> GPLGSSLFNSEEDVVKMSPLPTVENQFTPTTAWSTSVGSGIGNFYSNLHPALADNVVYAADRAGLVKALNADDGKEIWSVSLAEKDGWFSKEPALLSGGVTVSGGHVYIGSEKAQVYALNTSDGTVAWQTKVAGEALSRPVVSDGLVLIHTSNGQLQALNEADGAVKWTVNLDMPSLSLRGESAPTTAFGAAVVGGDNGRVSAVLMEQGQMIWQQRISQATGSTEIDRLSDVDTTPVVVNGVVFALAYNGNLTALDLRSGQIMWKRELGSVNDFIVDGNRIYLVDQNDRVMALTIDGGVTLWTQSDLLHRLLTS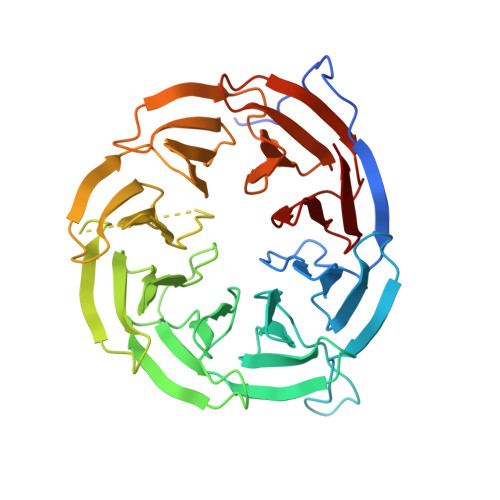PVLYNGNLVVGDSEGYLHWINVEDGRFVAQQKVDSSGFQTEPVAADGKLLIQAKDGTVYSITR>GRRKRTAVTGSQTALLLRAFEKDRFPGIAAREELARETGLPESRIQIWFQNRRARHPGQG[2x]

The HD2 domain folds into a global domain of three helices, α1–α3, respectively. The N-terminal poly-Arg/Lys motif, perpendicular to the helix α1, engages the DNA binding. In current HD2-DNAERG structure, the QNR motif is also the major DNA-code-reading module. Taken together, the new DUX4HD2-DNAERG structure shed new insight into the DUX4-DRE recognition: (1) DUX4 HD1-HD2 might bind preferentially to the repetitive DNA sequences containing 5′-GATXXGAT-3′, 5′-TAATXTAAT-3′ and 5-TGAT/TAAT-5′ (the complementary chain is underlined) motifs.

Furthermore, the GATXXGAT-like, TGAT-ATTA-like repeats are also frequently associated with wild type DUX4 and DUX4/IGH target genes. In order to gain more insight into the true nature of DUX4-DRE interaction, we have determined the structure of DUX4 HD2 bound with endogeneous ERG DNA sequences derived from the B-ALL patient RNA-seq and ChIP-seq analysis. The crystal of HD2-DREERG diffracted remarkably well (1.6 Å) compared with that of DUX4HD2–DREconsensus (2.6 Å). Consistent with previous report, one ERG DNA duplex can bind to two HD2 molecules. Unlike the previous 2.6 Å HD2-DREconsensue structure, the electron density map of ERG DNA is of high quality (1.6 Å) and allows clear registration of ERG sequences, 5′-T1GATGAGATT11-3′/3′-A1CTACTCTAA11-5′. The electron density map of the last pair of nucleotides, T11 and A11, are disordered and hence not available for model building. In this structure, the Arg95 and Arg98 side-chains dip into the minor groove. In particular, Arg98 forms a hydrogen bond with the hydroxyl group of T1 nucleotide. To our surprise, the Asn144 and Arg148 form two pairs of hydrogen bond with the G2 and A3 nucleotide. Consistently with previous observation, the high-resolution DUX4HD2-DNAERG structure reveals an interesting Gln143-water-nucleotide network in the major groove. In this report, the 1.6 Å DUX4HD2-DNAERG structure demonstrates a strong association between DUX4 homeobox and TGAT.7-(3-methylphenyl)pyrazolo[1,5-a]pyrimidine-3-carboxamide | C14 H12 N4 O | 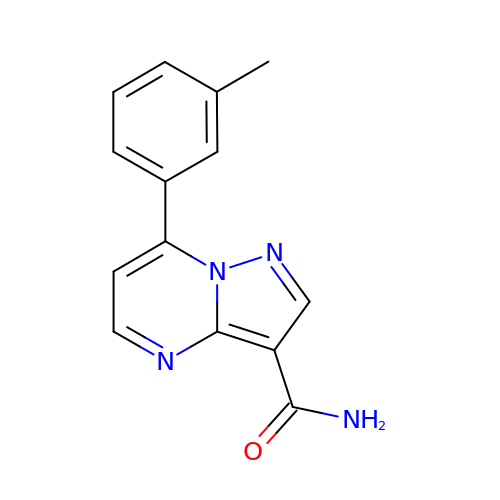HNKGGVGQAVODNJ-UHFFFAOYSA-N> GAMGSHMEFMDYDFKVKLSSERERVEDLFEYEGCKVGRGTYGHVYKAKRKDGKDDKDYALKQIEGTGISMSACREIALLRELKHPNVISLQKVFLSHADRKVWLLFDYAEHDLWHIIKFHRASKANKKPVQLPRGMVKSLLYQILDGIHYLHANWVLHRDLKPANILVMGEGPERGRVKIADMGFARLFNSPLKPLADLDPVVVTFWYRAPELLLGARHYTKAIDIWAIGCIFAELLTSEPIFHCRQEDIKTSNPYHHDQLDRIFNVMGFPADKDWEDIKKMPEHSTLMKDFRRNTYTNCSLIKYMEKHKVKPDSKAFHLLQKLLTMDPIK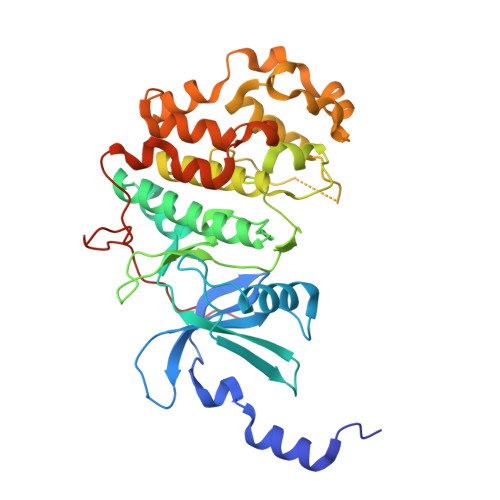RITSEQAMQDPYFLEDPLPTSDVFAGCQIPYPKREFLTEEEPDDKGDKK> NARFCILGSEAATRKHLPARNHCGLSDSSPQLWPEPDFRNPPRKASKASLDFKRYVTDRRLAETLAQIYLGKPSRPPHLLLECNPGPGILTQALLEAGAKVVALESDKTFIPHLESLGKNLDGKLRVIHCDFFKLDPRSGGVIKPPAMSSRGLFKNLGIEAVPWTADIPLKVVGMFPSRGEKRALWKLAYDLYSCTSIYKFGRIEVNMFIGEKEFQKLMADPGNPDLY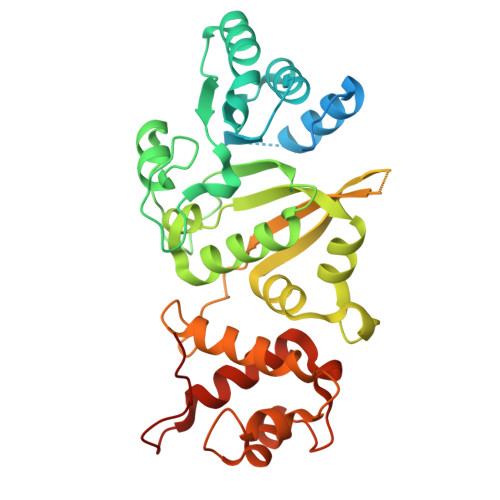HVLSVIWQLACEIKVLHMEPWSSFDIYTRKGPLENPKRRELLDQLQQKLYLIQMIPRQNLFTKNLTPMNYNIFFHLLKHCFGRRSATVIDHLRSLTPLDARDILMQIGKQEDEKVVNMHPQDFKTLFETIERSKDCAYKWLYDETLEDR>[2x]GSHMGGERTVTIRRQTVGGFGLSIKGGAEHNIPVVVSKISKEQRAELSGLLFIGDAILQINGINVRKCRHEEVVQVLRNAGEEVTLTVSFLKRAPGSAYGSVKAYTNFDAERDALNIETAIKTKGVDEVTIVNILTNRSNEQRQDIAFAYQRRTKKELASALKSALSGHLETVILGLLKTPAQYDASELKASMKGLGTDEDSLIEIICSRTNQELQEINRVYKEMYKTDL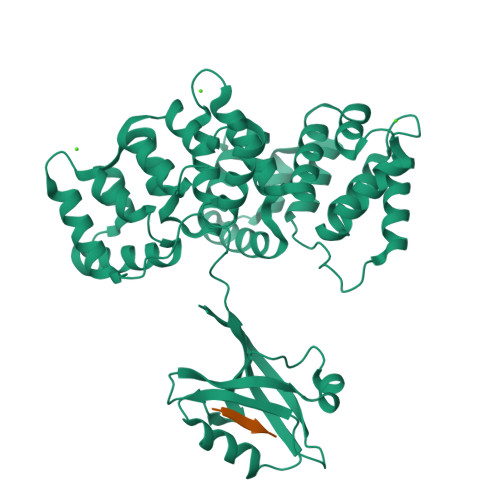EKDIISDTSGDFRKLMVALAKGRRAEDGSVIDYELIDQDARDLYDAGVKRKGTDVPKWISIMTERSVPHLQKVFDRYKSYSPYDMLESIRKEVKGDLENAFLNLVQCIQNKPLYFADRLYDSMKGKGTRDKVLIRIMVSRSEVDMLKIRSEFKRKYGKSLYYYIQQDTKGDYQKALLYLCGGDD;>EVEEFPETSV[2x]>[2x]MASMTGGQQMGRDEAGITGTWYNQLGSTFIVTAGADGALTGTYESAVGNAESRYVLTGRYDSAPATDGSGTALGWTVAWKNNYRNAHSATTWSGQYVGGAEARINTQWLLTYGTTEANAWESTLVGHDTFTKVKPSAASIDAAKKAGVNNGNPLDAVQQ

Introduction of a biotinylated monophosphine palladium complex within streptavidin affords an enantioselective artificial Suzukiase. ArMs result from the incorporation of an abiotic cofactor within a macromolecule (protein or oligonucleotide). Inspired by a seminal contribution by Whitesides in 1978,32 we report herein our effort to engineer an asymmetric artificial Suzukiase based on the biotin–streptavidin technology. In summary, incorporation of an electron-rich phosphino–palladium moiety within Sav affords an artificial Suzukiase for the synthesis of enantioenriched binaphthyls (up to 90% ee and 50 TONs for 2-methoxy-binaphthyl 8b).

To gain structural insight on the second coordination sphere around the Pd moiety, crystals of Sav S112Y–K121E were grown and soaked with a solution of 1 in DMSO (for details, see ESI†). In the resulting structure of complex 1·S112Y–K121E Sav, there is strong residual electron density in the 2Fo – Fc difference map in the biotin-binding vestibule. The Pd atom was unambiguously assigned as a strong peak in the difference map (12σ) with a corresponding peak in the anomalous difference map (8σ). The density map clearly highlights the presence of the phosphine ligand, the palladium, and the chloride (see ESI Fig. S5†). However, the cinnamyl ligand could not be resolved, likely due to disorder caused by ligand fluxionality. The amide linker exhibits two H-bonding interactions with the protein backbone: the amide nitrogen exhibits an H-bonding interaction with the side-chain of S88, and the carbonyl oxygen exhibits an H-bonding interaction with the backbone nitrogen of N49. The palladium atoms of two symmetry related-cofactors (face-to-face) are separated by 11.7 Å. The palladium was found in the vicinity of the O atoms of S112Y and K121E (Pd···O distance 6.4 Å and 7.1 Å respectively). Inspection of the X-ray structure of the active site of 1·S112Y–K121E shows that the Pd-phosphine ligand is effectively “locked” into place by the steric environment of the Sav protein, which is evidenced by the discrete atomic position of the Pd and P and their relatively low B-factors despite proximity to the solvent pocket. Furthermore, the conformation of Y112 is effectively locked in place by an H-bonding interaction of the sidechain oxygen with the backbone carbonyl of E121 (distance 2.88 Å), which would not be the case with the similarly large S112W mutation (entry 18).> DTVKIDANVN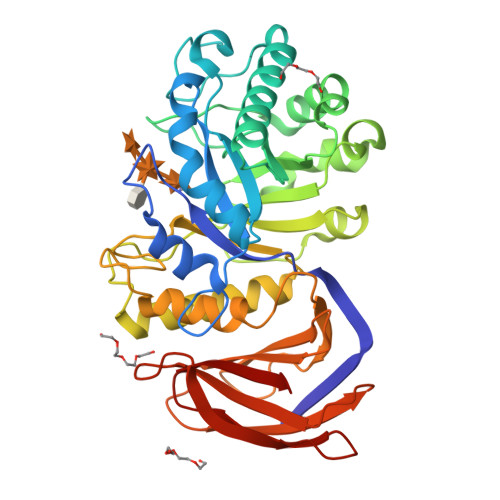YQIIQGFGGMSGVGWINDLTTEQINTAYGSGVGQIGLSIMRVRIDPDSSKWNIQLPSARQAVSLGAKIMATPWSPPAYMKSNNSLINGGRLLPANYSAYTSHLLDFSKYMQTNGAPLYAISIQNEPDWKPDYESCEWSGDEFKSYLKSQGSKFGSLKVIVAESLGFNPALTDPVLKDSDASKYVSIIGGHLYGTTPKPYPLAQNAGKQLWMTEHYVDSKQSANNWTSAIEVGTELNASMVSNYSAYVWWYIRRSYGLLTEDGKVSKRGYVMSQYARFVRPGALRIQATENPQSNVHLTAYKNTDGKMVIVAVNTNDSDQMLSLNISNANVTKFEKYSTSASLNVEYGGSSQVDSSGKATVWLNPLSVTTFVSK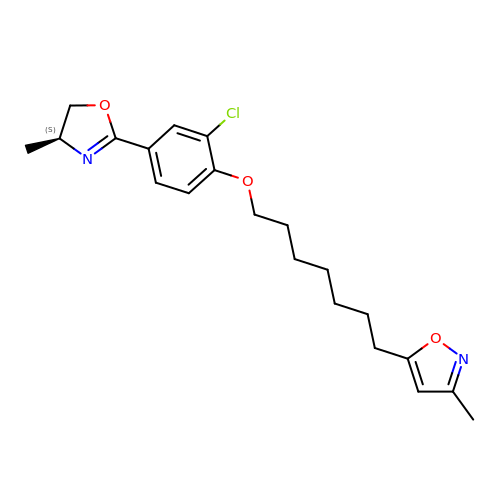5-(7-(6-CHLORO-4-(5-HYDRO-4-METHYL-2-OXAZOLYL)PHENOXY)HEPTYL)-3-METHYL ISOXAZOLE | C21 H27 Cl N2 O3 | WOJFAPUTPSWFLJ-INIZCTEOSA-N N-[(3S,4R,5S,6R)-4,5-dihydroxy-6-(hydroxymethyl)piperidin-3-yl]acetamide | C8 H16 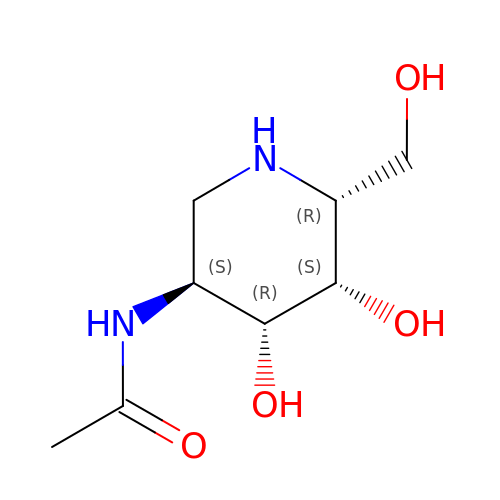N2 O4 | GBRAQQUMMCVTAV-OSMVPFSASA-N Uropathogenic Escherichia coli strains use filamentous type 1 pili to adhere to and invade uroepithelial cells. The pilus consists of a flexible tip fibrillum, formed by the adhesin FimH and the subunits FimG and FimF. The pilus rod is a helical assembly of up to 3000 copies of the main subunit FimA, terminated by a single copy of the subunit FimI that anchors the rod to the assembly platform FimD in the outer membrane. The assembly platform FimD in the outer membrane of uropathogenic E. coli is the catalyst of type 1 pilus assembly.

The assembly conditions were further optimized to produce a sample with an average pilus length suitable for cryo-EM, allowing us to determine the overall structure of the FimDHGFAnC complex to 4.1 Å resolution. The 3D-reconstruction of the complex (map I) revealed that the pilus rod sits at an angle on top of the usher. However, the rod was initially not well-resolved due to its flexible connection between subunit FimAn-1 occupying the pore and FimAn-2 emerging from the pore. To address this, multiple data processing strategies in single-particle analysis were employed, which significantly improved the resolution of both the pilus rod and the FimA-bound usher. Multi-body refinement in RELION-5.033,34 further enhanced the resolutions, yielding 3.6 Å for the pilus rod (body 1) and 3.9 Å for the assembly platform (body 2). By combining the maps of the two bodies, we constructed a composite map that includes both the assembly platform and pilus rod, which sits at an approximately 51° angle on top of the usher. Multi-body refinement provided insights into the movement of the pilus rod relative to the assembly platform. Although restrained by the rim of the β-barrel and the extracellular loops of FimD, principal component analysis revealed a twisting motion of up to 11°, as well as side-to-side and back-and-forth motions of up to 19° and 18°, respectively. This flexible connection likely enhances the range of the pilus, enabling it to bind mannose binding sites on the epithelial host cell surface more effectively. Importantly, it is only between FimAn-2 and FimAn-3 that the characteristic angle observed between adjacent FimA subunits within the mature pilus rod can finally be adopted.

>MAATTVNGGTVHFKGEVVNAACAVDAGSVDQTVQLGQVRTASLAQEGATSSAVGFNIQLNDCDTNVASKAAVAFLGTAIDAGHTNVLALQSSAAGSATNVGVQILDRTGAALTLDGATFSSETTLNNGTNTIPFQARYFATGAATPGAANADATFKVQYQ[10x]> MTTLADVKKRIGLKDEKQDEQLEEIIKSCESQLLSMLPIEVEQIPERFSYMIKEVAVKRYNRIGAEGMTSEAVDGRSNAYE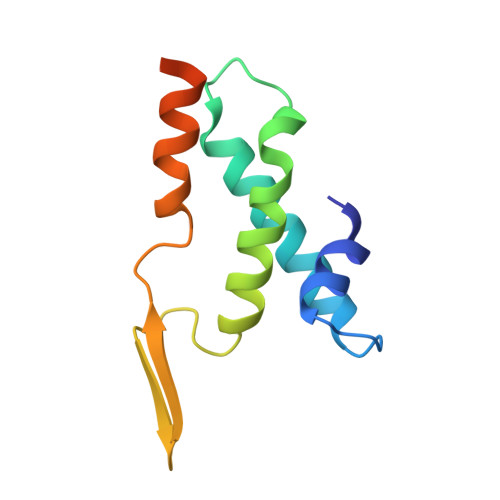LNDFKEYEAIIDNYFNARTRTKKGRAVFF> GIGTGFPFDPHYVEVLGERMHYVDVGPRDGTPVLFLHGNPTSSYVWRNIIPHVAPTHRCIAPDLIGMGKSDKPDLGYFFDDHVRFMDAFIEALGLEEVVLVIHAWGSALGFHWAKRNPERVKGIAFMEFIRPIPTWDEWPEFARETFQAFRTTDVGRKLIIDQNVFIEGTLPMGVVRPLTEVEMDHYREPFLNPVDREPLWRFPNELPIAGEPANIVALVEEYMDWLHQSPVPKLLFWGTPGVLIPPAEAARLAKSLPNCKAVDIGPGLNLLQEDNPDLIGSEIARWLSTLEI

The specific and covalent labeling of the protein HaloTag with fluorescent probes in living cells makes it a powerful tool for bioimaging. However, the irreversible attachment of the probe to HaloTag precludes imaging applications that require transient binding of the probe and comes with the risk of irreversible photobleaching. Here, we introduce exchangeable ligands for fluorescence labeling of HaloTag (xHTLs) that reversibly bind to HaloTag and that can be coupled to rhodamines of different colors. Here, we introduce exchangeable HaloTag Ligands (xHTLs) for the reversible fluorescence labeling of HaloTag7 with rhodamines, opening up new possibilities in bioimaging for a powerful labeling tool.

We then developed a second reversible labeling system with different ligand specificity, using a HaloTag7 mutant, for dual-color microscopy with xHTLs. Specifically, we mutated the active-site residue Asp106 in HaloTag7 to Ala (D106A), resulting in dHaloTag76. The loss of the interaction of the (trifluoromethyl)sulfonamide of xHTLs with D106 resulted in up to 57-fold lower affinities of dHaloTag7 for these probes compared to HaloTag7. We then found that primary hydroxy derivatives with different alkyl chain lengths (Hy4 and Hy5) displayed up to 108-fold higher binding affinity for dHaloTag7 over HaloTag7. Hy4 and Hy5 also possess fast non-covalent binding to dHaloTag7 and, coupled to appropriate fluorophores, fluorogenicity comparable to S5 probes. While the chloride forms hydrogen bonds with the W107 and N41 main chains, the water molecule occupies the space freed by the D106A mutation and interacts with the W107 and N41 side chains. Both chloride and water molecules form hydrogen bonds with the Hy5 ligand. Hy5-based xHTLs showed higher binding affinity than the corresponding Hy4-based xHTLs, which was required in the case of MaP555-Hy5 for selective staining of intracellular dHaloTag7. In in vitro titrations, probes based on Hy4, Hy5, or S5 had >50-fold higher affinities for their cognate HaloTag variant, whereas T5-based probes showed lower specificity. Furthermore, both PAINT and STED microscopy can be performed in dual color using pairs of xHTLs together with HaloTag7 and dHaloTag7.> MIVSAIAANALLESVTKFHCGVIYDYSTAEYVSYRPSDFGAYLDALEAEVARGGLIVFHNGHKYDVPALTKLAKLQLNREFHLPRENCIDTLVLSRLIHSNLKDTDMGLLRSGKLPGKRFGSHALEAWGYRLGEMKGEYKDDFKRMLEEQGEEYVDGMEWWNFNEEMMDYNVQDVVVTKALLEKLLSDKHYFPPEIDFTDVGYTTFWSESLEAVDIEHRAAWLLAKQERNGFPFDTKAIEELYVELAARRSELLRKLTETFGSWYQPKGGTEMFCHPRTGKPLPKYPRIKTPKVGGIFKKPKNKAQREGREPCELDTREYVAGAPYTPVEHVVFNPSSRDHIQKKLQEAGWVPTKYTDKGAPVVDDEVLEGVRVDDPEKQAAIDLIKEYLMIQKRIGQSAEGDKAWLRYVAEDGKIHGSVNPNGAVTGRATHAFPNLAQIPGVRSPYGEQCRAAFGAEHHLDGITGKPWVQAGIDASGLELRCLAHFMARFDNGEYAHEILNGDIHTKNQIAAELPTRDNAKTFIYGFLYGAGDEKIGQIVGAGKERGKELKKKFLENTPAIAALRESIQQTLVESSQWVAGEQ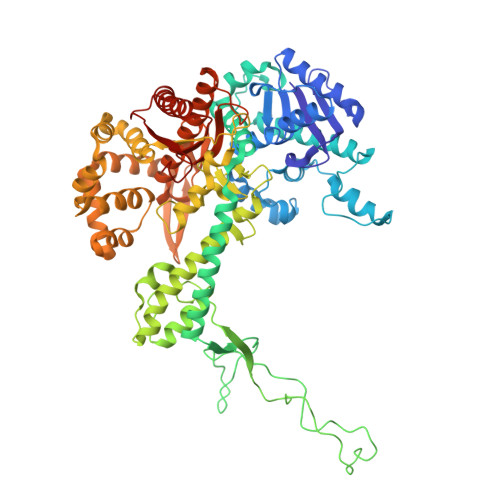QVKWKRRWIKGLDGRKVHVRSPHAALNTLLQSAGALICKLWIIKTEEMLVEKGLKHGWDGDFAYMAWVHDEIQVGCRTEEIAQVVIETAQEAMRWVGDHWNFRCLLDTEGKMGPNWAICH>[2x]MFEQRVNSDVLTVSTVNSQDQ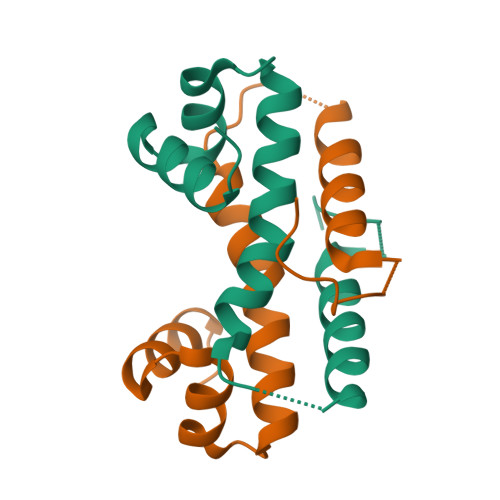VTQKPLRDSVKQALKNYFAQLNGQDVNDLYELVLAEVEQPLLDMVMQYTRANQTRAALMMGINRGTLRKKLKKYGMN>[2x]RRRSGSLVYQKRRRRLLPFVSSEDPAQRLKQMGTL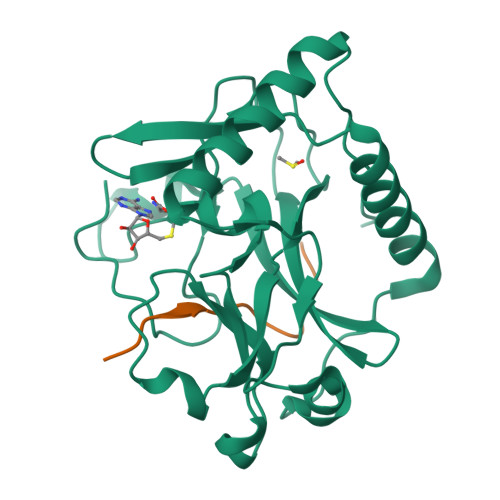ASALTELQMEFSDDLTYSSGMAPRSANQARFEEGGMQVLTKEDIETLEQCRAMCKRGDCPPLLVVFDSREGFTVEADGQIKDMTFIAEYTGDVDYIRNREHDDCDSMMTLLLAKDPSKSLVICPDKRGNIARFISGINNHTLDGKKKQNCKCVRYSVNGECRVFLVATRDIAKGERLYYDYNGYEHEYPTQHFV;>KAARKSAPATGGVK[2x]>[2x]MTDFLAGIRIVGEDKNGMTNQITGVI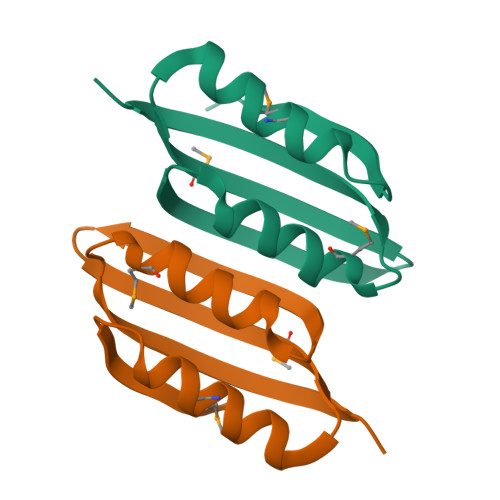SKFDTNIRTIVLNAKDGIFTCNLMIFVKNTDKLTTLMDKLRKVQGVFTVERLSNLEHHHHHH>[4x]KIIMISGANSGIGHACIKYFLEKSFHVIALDINNNNLIDYMKTDMPLKVVQIDLSNSEAIHNLFTQLDLEKLSPDILINAAGIREITPVLHLSDDMFKKVIDVNLVAPFILSREVAKRWCESKIKGCIVNIASVSGLMAKPERAAYVASKHALIGLTKQMAMEFGKQNIRVNSISPGVIRTELTEEYFSNKALMSMIKSNQSLDTWGLPQDIVSCIEYLISDQARFITGSNFVIDGGQTAGKNLLEKGELNSKLEGKPIPNPLLGLDSTRTGHHHHHH

HILDH belongs to the short-chain dehydrogenase/reductase (SDR) superfamily. HILDH reduces the racemic AMKP to (2S,3R,4S)-4-HIL and the other seven stereoisomers of 4-HIL in an NADH-dependent manner, suggesting that HILDH has nearly no stereoselectivity with AMKP. HILDH forms a tetrameric structure, and each subunit consists of seven α-helices, seven β-strands and three 310-helices.

To explain the structural mechanism of the high selectivity of the E144K/W242Q mutant toward (2S,3R,4S)-4-HIL, we solved the crystal structure of HILDHE144K/W242Q in complex with NADH and succinate at 1.90 Å resolution. The electron densities of succinate molecules, K144 and Q242 are clearly observed in the active site of all four subunits to HILDHE144K/W242Q. However, in the crystal structure of HILDHE144K/W242Q, the electron density of K144 is clearly observed; the side-chain configuration of K144 is fixed by a hydrogen-bonding network with succinate, Q242 and a water molecule. The side-chain amino group of K144 forms a hydrogen bond with the side-chain amide oxygen of Q242. A water molecule is trapped by the side-chain amino group of K144, the side-chain amide nitrogen of Q242 and the C1-carboxy group of succinate. The succinate molecule bound to the active site of HILDHE144K/W242Q is recognized by 7 residues of HILDHE144K/W242Q. The C4-carboxy group interacts with S137, S139, K144 and Y150. The carboxy group at C-1 is recognized by R88, R147 and Y191. The binding mode of succinate in the HILDHE144K/W242Q mutant mimics that of the 4R form of 4-HIL, as well as the wild-type structure. The O4 atom is recognized by S139 and K144, but not when the O4 atom is substituted by a methyl group in the 4R form of 4-HIL, the hydrophobic methyl group would hardly be adopted by hydrophilic S139 and K144.> MEGSTGFDGDATTFFAPDAVFGDRVRRFQEFLDTFTSYRDSVRSIQVYNSNNAANYNDDQDDADERDLLGDDDGDDLEKEKKAASSTSLNILPHRIIISLDDLREFDRSFWSGILVEPAYFIPPAEKALTDLADSMDDVPHPNASAVSSRHPWKLSFKGSFGAHALSPRTLTAQHLNKLVSVEGIVTKTSLVRPKLIRSVHYAAKTGRFHYRDYTDATTTLTTRIPTPAIYPTEDTEGNKLTTEYGYSTFIDHQRITVQEMPEMAPAGQLPRSIDVILDDDLVDKTKPGDRVNVVGVFKSLGAGGMNQSNSNTLIGFKTLILGNTVYPLHARSTGVAARQMLTDFDIRNINKLSKKKDIFDILSQSLAPSIYGHDHIKKAILLMLMGGVEKNLENGSHLRGDINILMVGDPSTAKSQLLRFVLNTASLAIATTGRGSSGVGLTAAVTTDRETGERRLEAGAMVLADRGVVCIDEFDKMTDVDRVAIHEVMEQQTVTIAKAGIHTTLNARCSVIAAANPVFGQYDVNRDPHQNIALPDSLLSRFDLLFVVT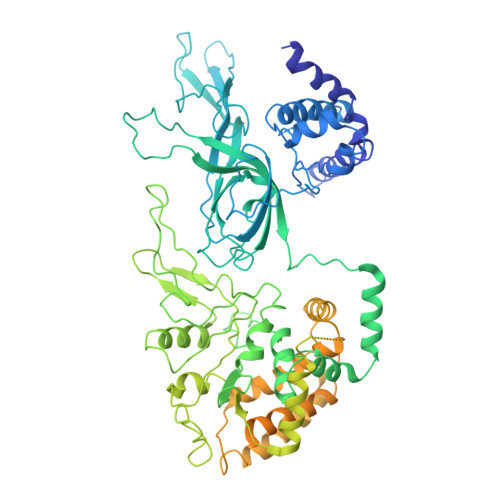DDINEIRDRSISEHVLRTHRYLPPGYLEGEPVRERLNLSLAVGEDADINPEEHSNSGAGVENEGEDDEDHVFEKFNPLLQAGAKLAKNKGNYNGTEIPKLVTIPFLRKYVQYAKERVIPQLTQEAINVIVKNYTDLRNDDNTKKSPITARTLETLIRLATAHAKVRLSKTVNKVDAKVAANLLRFALLGEDIGNDIDEEESEYEEALSKRSPQKSPKKRQRVRQPASNSGSPIKSTPRRSTASSVNATPSSARRILRFQDDEQNAGEDDNDIMSPLPADEEAELQRRLQLGLRVSPRRREHLHAPEEGSSGPLTEVGTPRLPNVSSAGQDDEQQQSVISFDNVEPGTISTGRLSLISGIIARLMQTEIFEEESYPVASLFERINEELPEEEKFSAQEYLAGLKIMSDRNNLMVADDKVWRV> MKRKPNSNQNNNNNRGNGNGLRRVRGGRVSRRRVVINQSNQSMPVTSNGAPLQALTSYSRPNVNKISRLGPDSDFLTSVVAKASTSIVTPADRILVKQPLSASSFPGTRITGLSSYWERYKWLSAVARYVPAVPNTVACQFVMYIDTDPLDDPSNISDDNQIVRQAVSQAGSNQFNFNTSKTVPLIVRADNQYYYTGVDKQNLRFSLQGILYIIQVTDLINFNGELITQDLTCGSLFLDWLVNFSIPQINPTSLTDVRVDKAVNFIKPEVSGVAEIQTVTGLSPSTSYLLTPAFLEQNFQSEAGIYILSATPVEGEGTISINMDPTVTTVSGFIKVKTDTFGTFDLSVVLTTASKKQTTGFNI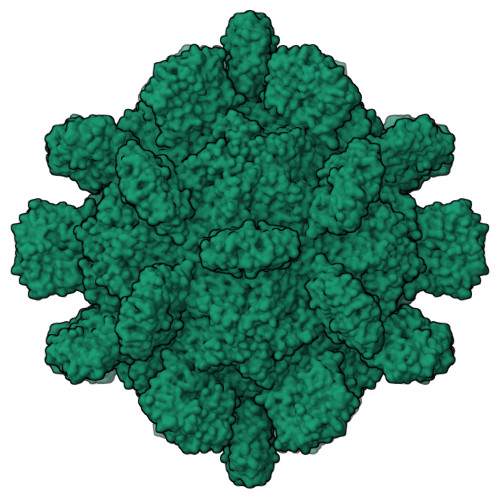IAATS4-HYDROXYBUTAN-1-AMINIUM | C4 H12 N O | 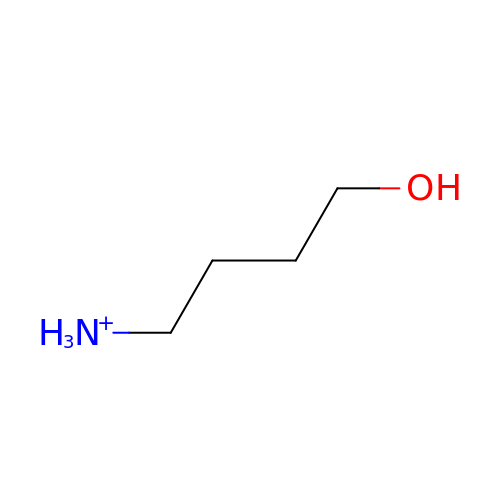BLFRQYKZFKYQLO-UHFFFAOYSA-O> SGAKDSG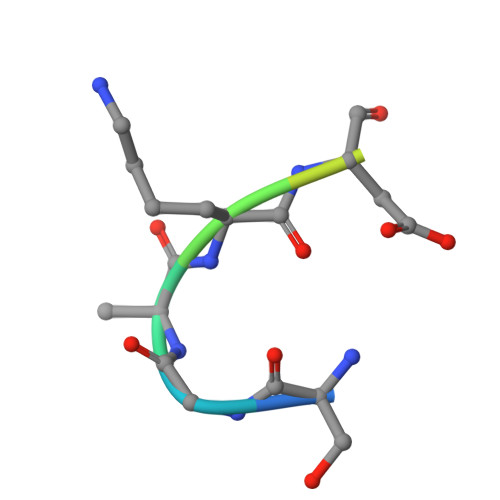SLR> MIKATYSSAKDFYSLLSGLLKVTDEIILNFTEDSIFSRYLTDDKVLMVIFKIPKEYLEDYTIDKPLGIKININDLKKILGKAKSKSATVTLEETEAGLKVTVRDEKTGTRSNIYIKGEKTSIDQLTEPKVNLSVTFTTDGDVLKDIARDLSLVGE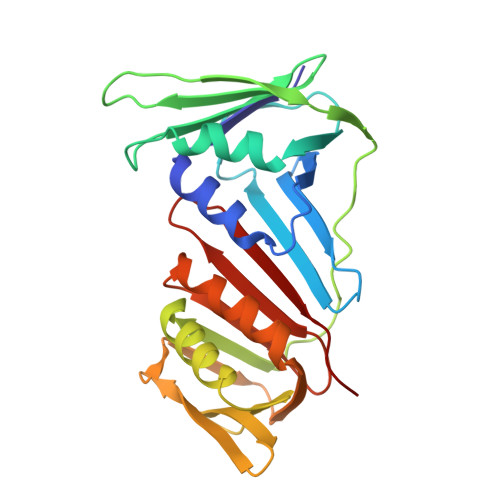EVEISADENTVTLSTEEAGRTYKSLLKQDKPLKSLNVESPSKAVYSIEVLKDVFKVTSISQNVTVGFGNNIPMKIEVPTDSGGQLIFWIAPRL>DCYTELEKAVIVLVENFYKYVSKYSLVKNKISKSSFREMLQKELNHMLSDTGNRKAADKLIQNLDANHDGRISFDEYWTLIGGITGPIAKLIHE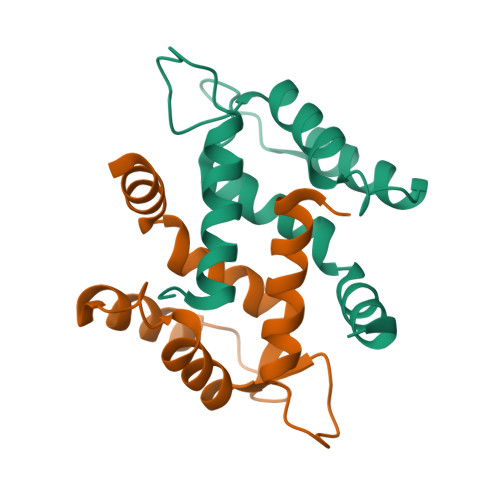QEQQSS[4x]> CACGAGCCTGATCGGACAAGATCCG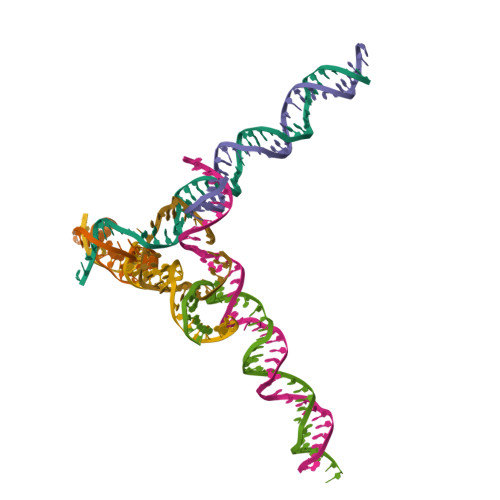CTAGCGAGTTAGCCTAG;> GAGCAGCCTGTACGGACATCAGTCTCTGCTAGATCGTCAGCA;> AACCTACCTGGCAGGACGACTGCCTATGCTA;> TGCTAGGCTAACTCGCTAGCGGATCTTGTGGCTGC;> TTTAGCATAGGCAGTCGTGGCTCG;> TCTGCTGACGATCTAGCAGAGACTGATGTGGTAGG;> CACCGATCACCTGCCACCGTA>[2x]MKKIEHKMVAVNGLNMHLAELGEGPTILFIHGFPELWYSWRHQMVYLAERGYRAVAPDLRGYGDTTGAPLNDPSKFSILHLVGDVVALLEAIAP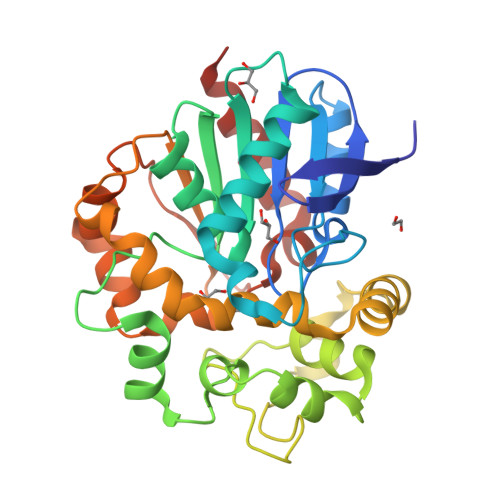NEEKVFVVAHDWGALIAWHLCLFRPDKVKALVNLSVHFSKRNPKMNKVEGLKAIYGEDHYVSRFQVPGEIEAEFAPIGAKSVLKKILTYRDPAPFYFPKGKGLEAIPDAPVALSSWLSEEELDYYANKFEQTGFTGAVNYYRALPINWELTAPWTGAQVKVPTKFIVGEFDLVYHIPGAKEYIHNGGFKKDVPLLEEVVVLEGAAHFVSQERPHEISKHIYDFIQKFTSHHHHH>[2x]GSHMRLGAQSIQPTANLDRTDDLVYLNVMELVRAVLELKNELAQLPPEGYVVV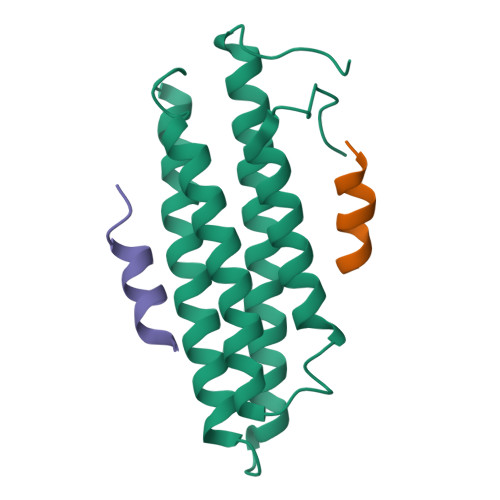VKNVGLTLRKLIGSVDDLLPSLPSSSRTEIEGTQKLLNKDLAELINKMRLAQQNAVTSLSEECKRQMLTASHTLAVDAKNLLDAVDQAKVLANLAHPPAE;>ATRELDELMASLS[4x]> EKLVQPTPLLLSLLKSAGAQKETFTMKEVLYHLGQYIMAKQLYDEKQQHIVHCSNDPLGELFGVQEFSVKEHRRIYA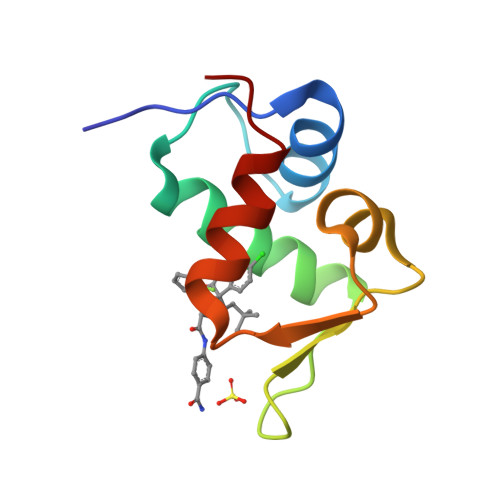MISRNLVS>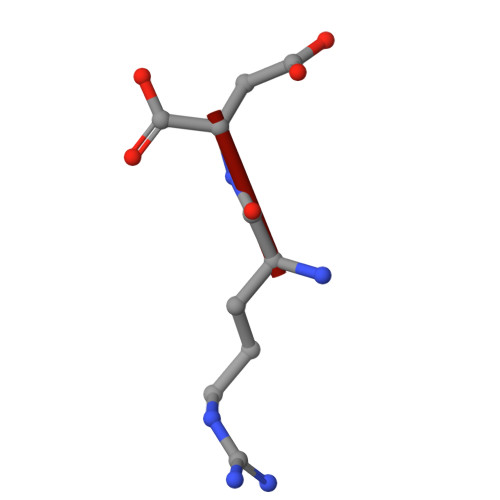 RD2,2,2-trifluoromethyl acetophenone hydrate | C8 H7 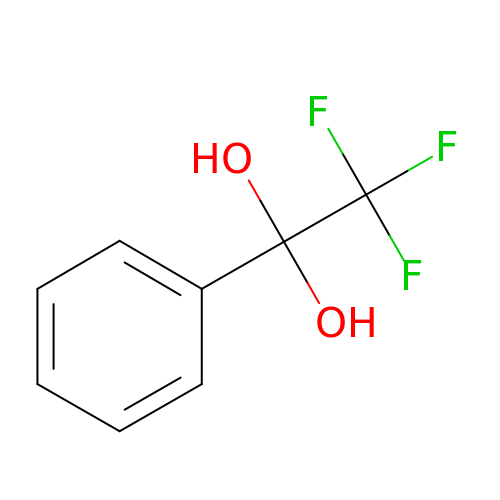F3 O2 | APDULARNYREANX-UHFFFAOYSA-N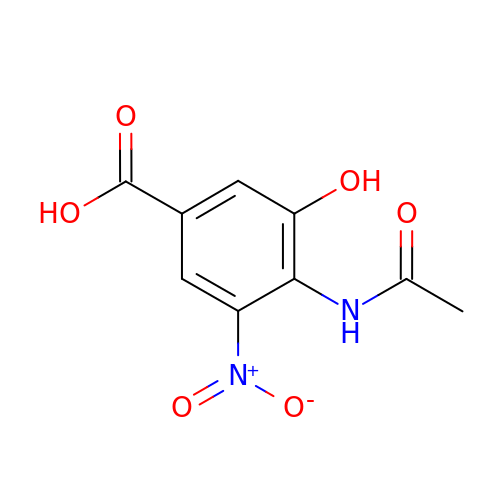4-(ACETYLAMINO)-3-HYDROXY-5-NITROBENZOIC ACID | C9 H8 N2 O6 | JIDRTCHFBHJIDG-UHFFFAOYSA-N Aerolysin is a β-pore-forming toxin produced by most Aeromonas bacteria, which has attracted large attention in the field of nanopore sensing due to its narrow and charged pore lumen. Pore-forming toxins (PFTs) are important virulence factors of many pathogenic bacteria, which are secreted in a soluble form and upon host membrane binding, they oligomerize into transmembrane pores undergoing a complex structural reorganization. Domains 3 and 4 form the 120 Å long 14-stranded β-barrel, with each protomer contributing two antiparallel β-strands. Four distinct constriction rings, two at each end of the pore, were identified from the structures and confirmed by MD simulation.

We have recently demonstrated that the K238A mutation enhances the sensing capabilities and sensitivity due to a longer dwell time of the analyte in the pore. To unravel the structural basis for this improved performance, we have solved the structure of the K238A mutant in SMALP obtaining a density map at 2.2 Å. The structures of the WT and mutant in SMALP are highly similar, exhibiting an RMSD of 0.92 Å and comparable pore cavities shown both from the raw structure and in MD simulations. Upon closer examination of the mutant structure, it becomes evident that the K238A mutation induces widening of the third constriction ring. This is attributed to the substitution of lysines with smaller alanine residue. In contrast to previous suggestions that the K238A mutation alters the analyte dwell time by decreasing the diameter of the constriction formed by R220,13 these structures reveal that all other constriction rings remain unaffected. Notably, for this mutant, we did observe a narrower water density from the MD simulation at R220, which is the same as previous MD results. The new structures indicate that the K238A mutation may influence the pore’s rigidity as it disrupts salt–bridge interactions between K238 and E258 within the barrel. A comparison of the ionic current response to different voltages revealed that the MD simulations in DPhPC bilayers based on the new K238A aerolysin structure solved in SMALPs yielded results that very closely aligned with the experimental data and are better than previous estimations, especially when negative voltage is applied.

>AEPVYPDQLRLFSLGQGVCGDKYRPVNREEAQSVKSNIVGMMGQWQISGLANGWVIMGPGYNGEIKPGTASNTWCYPTNPVTGEIPTLSALDIPDGDEVDVQWRLVHDSANFIKPTSYLAHYLGYAWVGGNHSQYVGEDMDVTRDGDGWVIRGNNDGGCDGYRCGDKTAIKVSNFAYNLDPDSFKHGDVTQSDRQLVKTVVGWAVNDSDTPQSGYDVTLRYDTATNWSKTNTYGLSEAVTTKNKFKWPLVGETELSIEIAANQSWASQNGGSTTTSLSQSVRPTVPARSKIPVKIELYKADISYPYEFKADVSYDLTLSGFLRWGGNAWYTHPDNRPNWNHTFVIGPYKDKASSIRYQWDKRYIPGEVKWWDWNWTIQQNGLSTMQNNLARVLRPVRAGITGDFSAESQFAGNIEIGAPVPLAA[7x]>[4x]MPKRTDIKSILILGAGPIVIGQACEFDYSGAQACKALREEGYRVILVNSNPATIMTDPEMADATYIEPIHWEVVRKIIEKERPDAVLPTMGGQTALNCALELERQGVLEEFGVTMIGATADAIDKAEDRRRFDVAMKKIGLETARSGIAHTMEEALAVAADVGFPCIIRPSFTMGGSGGGIAYNREEFEEICARGLDLSPTKELLIDESLIGWKEYEMEVVRDKNDNCIIVCSIENFDAMGIHTGDSITVAPAQTLTDKEYQIMRNASMAVLREIGVETGGSNVQFAVNPKNGRLIVIEMNPRVSRSSALASKATGFPIAKVAAKLAVGYTLDELMNDITGGRTPASFEPSIDYVVTKIPRFNFEKFAGANDRLTTQMKSVGEVMAIGRTQQESLQKALRGLEVGATGFDPKVSLDDPEALTKIRRELKDAGADRIWYIADAFRAGLSVDGVFNLTNIDRWFLVQIEELVRLEEKVAEVGITGLNADFLRQLKRKGFADARLAKLAGVREAEIRKLRDQYDLHPVYKRVDTCAAEFATDTAYMYSTYEEECEANPSTDREKIMVLGGGPNRIGQGIEFDYCCVHASLALREDGYETIMVNCNPETVSTDYDTSDRLYFEPVTLEDVLEIVRIEKPKGVIVQYGGQTPLKLARALEAAGVPVIGTSPDAIDRAEDRERFQHAVERLKLKQPANATVTAIEMAVEKAKEIGYPLVVRPSYVLGGRAMEIVYDEADLRRYFQTAVSVSNDAPVLLDHFLDDAVEVDVDAICDGEMVLIGGIMEHIEQAGVHSGDSACSLPAYTLSQEIQDVMRQQVQKLAFELQVRGLMNVQFAVKNNEVYLIEVNPRAARTVPFVSKATGVPLAKVAARVMAGKSLAEQGVTKEVIPPYYSVKEVVLPF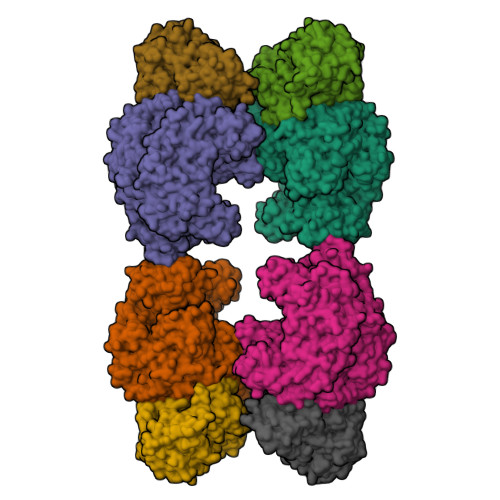NKFPGVDPLLGPEMRSTGEVMGVGRTFAEAFAKAQLGSNSTMKKHGRALLSVREGDKERVVDLAAKLLKQGFELDATHGTAIVLGEAGINPRLVNKVHEGRPHIQDRIKNGEYTYIINTTSGRRAIEDSRVIRRSALQYKVHYDTTLNGGFATAMALNADATEKVISVQEMHAQIK;>[4x]MIKSALLVLEDGTQFHGRAIGATGSAVGEVVFNTSMTGYQEILTDPSYSRQIVTLTYPHIGNVGTNDADEESSQVHAQGLVIRDLPLIASNFRNTEDLSSYLKRHNIVAIADIDTRKLTRLLREKGAQNGCIIAGDNPDAALALEKARAFPGLNGMDLAKEVTTAEAYSWTQGSWTLTGGLPEAKKEDELPFHVVAYDFGAKRNILRMLVDRGCRLTIVPAQTSAEDVLKMNPDGIFLSNGPGDPAPDDYAITAIQKFLETDIPVFGICLGHQLLALASGAKTVKMKFGHHGGNHPVKDVEKNVVMITAQNHGFAVDEATLPANLRVTHKSLFDGTLQGIHRTDKPAFSFQGHPEASPGPHDAAPLFDHFIELIEQYRKTAK> MAFQNDAKANFPDYANHGCVVGRHLNFEMYQRLFGKKTAHGVTVDKVIQPSVDNFGNCIGLIAGDEESYEVFKELFDAVINEK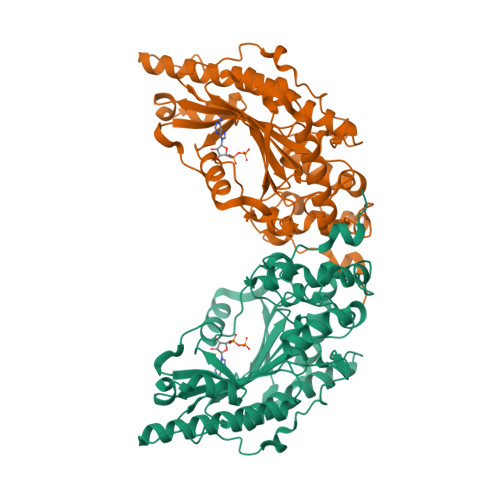HKGFGPNDSQPAPDLDASKLVGGQFDEKYVKSCRIRTGRGIRGLCYPPSCTRGERREVERVITTALAGLSGDLSGTYYPLSKMTPEQENQLIADHFLFQKPTGHLMVNSASVRDWPDARGIWHNNEKTFLIWINEEDHMRVISMQKGGNVKAVFERFGRGLNAIAEQMKKNGREYMWNQRLGYLCACPSNLGTGLRASVHVQLHQLSKHPKFEDIVVALQLQKRGTGGEHTAAVDDVYDISNAARLKKSEREFVQLLIDGVKKLIDMEQALEAGKSIDDLIPA>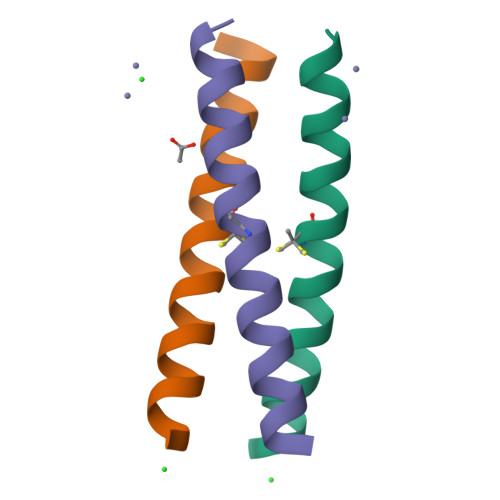[3x]XEWEALEKKLAALESKXQALEKKLEALEHGX> ASWSHPQFEKGAMSDTVIERHADTAALVAAAGDRLVDAISSAIGERGQATIVLTGGGTGIGLLKRVRERSGEIDWSKVHIYWGDER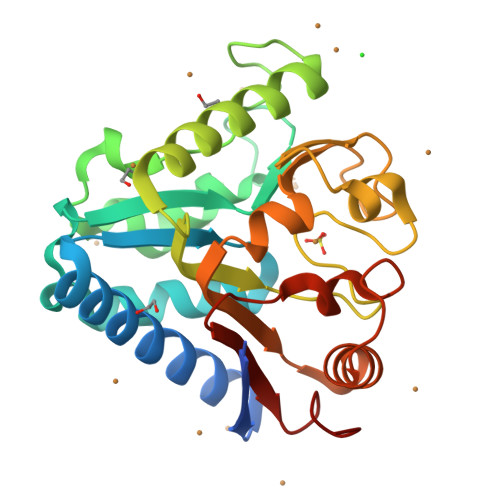FVPQDDDERNDKQAREALLDHIGIPPVNVHAMAASDGEFGDDLEAAAAGYAQLLSADFDSSVPGFDVHLLGMGGEGHVNSLFPDTDAVRETERLVVGVSDSPKPPPRRITLTLPAVQNSREVWLVVSGEAKADAVAAAVGGADPVDIPAAGAVGRERTVWLVDEAAAAKL> MLGTGPAAATTAATTSXXXXXXXXXXXXXXSRNEETXXXXXXXXXXXXXXXXXEMSQEESTRFYDQLNHHIFELVSSSDANERKGGILAIASLIGVEGGNATRIGRFANYLRNLLPSNDPVVMEMASKAIGRLAMAGDTFTAEYVEFEVKRALEWLGADRNEGRRHAAVLVLRELAISVPTFFFQQVQPFFDNIFVAVWDPKQAIREGAVAALRACLILTTQREPKEMQKPQWYRHTFEEAEKGFDETLAKEKGMNRDDRIHGALLILNELVRISSMEGERLREEMEEITQQQLVHDKYCKDLMGFGTKPRHITPFTSFQAVQPQQSNALVGLLGYSSHQGLMGFGTSPSPAKSTXXXXXXXXXXXXXXXXXXXXXXXXXRNSKNSLIQMTILNLLPRLAAFRPSAFTDTQYLQDTMNHVLSCVKKEKERTAAFQALGLLSVAVRSEFKVYLPRVLDIIRAALPPKDFAHKRQKAMQVDATVFTCISMLARAMGPGIQQDIKELLEPMLAVGLSPALTAVLYDLSRQIPQLKKDIQDGLLKMLSLVLMHKPLRHPGMPKGLAHQLASPGLTTLPEASDVGSITLALRTLGSFEFEGHSLTQFVRHCADHFLNSEHKEIRMEAARTCSRLLTPSIHLISGHAHVVSQTAVQVVADVLSKLLVVGITDPDPDIRYCVLASLDERFDAHLAQAENLQALFVALNDQVFEIRELAICTVGRLSSMNPAFVMPFLRKMLIQILTELEHSGIGRIKEQSARMLGHLVSNAPRLIRPYMEPILKALILKLKDPDPDPNPGVINNVLATIGELAQVSGLEMRKWVDELFIIIMDMLQDSSLLAKRQVALWTLGQLVASTGYVVEPYRKYPTLLEVLLNFLKTEQNQGTRREAIRVLGLLGALDPYKHKVNIGMIDQSRDASAVSLSESKSSQDSSDYSTSEMLVNMGNLPLDEFYPAVSMVALMRIFRDQSLSHHHTMVVQAITFIFKSLGLKCVQFLPQVMPTFLNVIRVCDGAIREFLFQQLGMLVSFVKSHIRPYMDEIVTLMREFWVMNTSIQSTIILLIEQIVVALGGEFKLYLPQLIPHMLRVFMHDNSPGRIVSIKLLAAIQLFGANLDDYLHLLLPPIVKLFDAPEAPLPSRKAALETVDRLTESLDFTDYASRIIHPIVRTLDQSPELRSTAMDTLSSLVFQLGKKYQIFIPMVNKVLVRHRINHQRYDVLICRIVKGYTLADEEEDPLIYQHRMLRSGQGDALASGPVETGPMKKLHVSTINLQKAWGAARRVSKDDWLEWLRRLSLELLKDSSSPSLRSCWALAQAYNPMARDLFNAAFVSCWSELNEDQQDELIRSIELALTSQDIAEVTQTLLNLAEFMEHSDKGPLPLRDDNGIVLLGERAAKCRAYAKALHYKELEFQKGPTPAILESLISINNKLQQPEAAAGVLEYAMKHFGELEIQATWYEKLHEWEDALVAYDKKMDTNKDDPELMLGRMRCLEALGEWGQLHQQCCEKWTLVNDETQAKMARMAAAAAWGLGQWDSMEEYTCMIPRDTHDGAFYRAVLALHQDLFSLAQQCIDKARDLLDAELTAMAGESYSRAYGAMVSCHMLSELEEVIQYKLVPERREIIRQIWWERLQGCQRIVEDWQKILMVRSLVVSPHEDMRTWLKYASLCGKSGRLALAHKTLVLLLGVDPSRQLDHPLPTVHPQVTYAYMKNMWKSARKIDAFQHMQHFVQTMQQQAQHAIATEDQQHKQELHKLMARCFLKLGEWQLNLQGINESTIPKVLQYYSAATEHDRSWYKAWHAWAVMNFEAVLHYKHQNQARDEKKKLRHASGANITNATTAATTAATATTTASTEGSNSESEAESTENSPTPSPLQKKVTEDLSKTLLMYTVPAVQGFFRSISLSRGNNLQDTLRVLTLWFDYGHWPDVNEALVEGVKAIQIDTWLQVIPQLIARIDTPRPLVGRLIHQLLTDIGRYHPQALIYPLTVASKSTTTARHNAANKILKNMCEHSNTLVQQAMMVSEELIRVAILWHEMWHEGLEEASRLYFGERNVKGMFEVLEPLHAMMERGPQTLKETSFNQAYGRDLMEA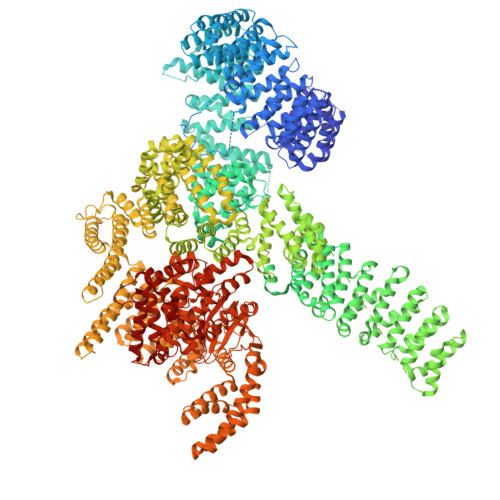QEWCRKYMKSGNVKDLTQAWDLYYHVFRRISKQLPQLTSLELQYVSPKLLMCRDLELAVPGTYDPNQPIIRIQSIAPSLQVITSKQRPRKLTLMGSNGHEFVFLLKGHEDLRQDERVMQLFGLVNTLLANDPTSLRKNLSIQRYAVIPLSTNSGLIGWVPHCDTLHALIRDYREKKKILLNIEHRIMLRMAPDYDHLTLMQKVEVFEHAVNNTAGDDLAKLLWLKSPSSEVWFDRRTNYTRSLAVMSMVGYILGLGDRHPSNLMLDRLSGKILHIDFGDCFEVAMTREKFPEKIPFRLTRMLTNAMEVTGLDGNYRITCHTVMEVLREHKDSVMAVLEAFVYDPLLNWRLMDTNTKGNKRSRTRTDSYSAGQSVEILDGVELGEPAHKKTGTTVPESIHSFIGDGLVKPEALNKKAIQIINRVRDKLTGRDFSHDDTLDVPTQVELLIKQATSHENLCQCYIGWCPFW>APVPVTKLVCDGDTYKCTA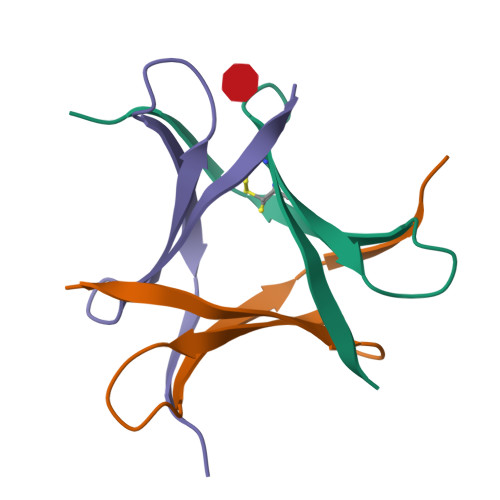YLDYGDGKWVAQWDTAVFHTT[6x]>[2x]MPTKKQKSKSKLKPFFALVRRTNPSYGKLAFALALSVVTTLVSLLIPLLTKQLVDGFSMSNLSGTQIGLIALVFFVQAGLSAYATYALNYNGQKIISGLRELLWKKLIKLPVSYFDTNASGETVSRVTNDTMVVKELITTHISGFITGIISVIGSLTILFIMNWKLTLLVLVVVPLAALILVPIGRKMFSISRETQDETARFTGLLNQILPEIRLVKASNAEDVEYGRGKMGISSLFKLGVREAKVQSLVGPLISLVLMAALVAVIGYGGMQVSSGELTAGALVAFILYLFQIIMPMGQITTFFTQLQKSIGATERMIEILAEEEEDTVTGKQIENAHLPIQLDRVSFGYKPDQLILKEVSAVIEAGKVTAIVGPSGGGKTTLFKLLERFYSPTAGTIRLGDEPVDTYSLESWREHIGYVSQESPLMSGTIRENICYGLERDVTDAEIEKAAEMAYALNFIKELPNQFDTEVGERGIMLSGGQRQRIAIARALLRN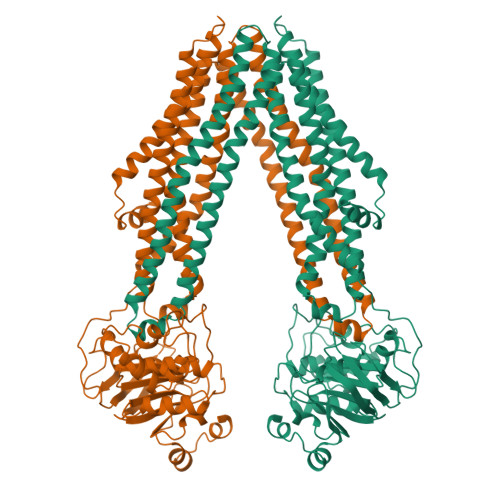PSILMLDEATSSLDSQSEKSVQQALEVLMEGRTTIVIAHRLSTVVDADQLLFVEKGEITGRGTHHELMASHGLYRDFAEQQLKMNADLENKAGVDKLAAALEHHHHHH> LEEHYYSRKTCGSGGGLSVQRTGYPQTDPPVFKAVNSFERAPLIVGDHVHSLPYWSRKITLECTPYPFTLRWEGGVHKDGIPDKVPHPSCDPGSELVSYTHSREVDCERFIGPVPSSFTDPKVTSAQWKFLEDMADMKALADLNKSLVNLPMLYKERRETLKMVGNRLGGLVRVAHAAQDRDLKRYFKARRKDRRKVAEEVANGHLELIFGWLPLIGELEGAIEYAELPDLDFIRCHGLHTLVLQSTPWDNSVDVRSYPNWERAAGTRITGSVRTRGVVESRASVRTALRFNLETSLAGDARRLGFEPISTTYDMIPLSFVVGWFSNFDKYVRTLAPLIGVTFETGSQNRRTTCELVGCTRFYPRTVSPP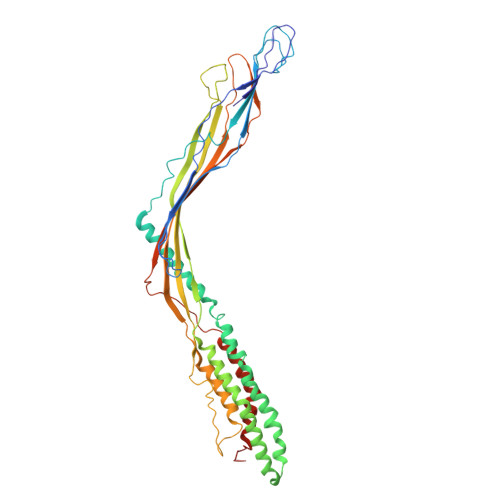SGWFARWKDFPDGSLSEVSGLRRTDIRSVLSTLPDPDVRFHADVGLFEISAGISLLAQRYLKPLQRLLKRKSFFYGRT>[2x]KKQTQRNVFRCNVIGVKNCGKSGVLQALLGRNLMRQKKIREDHKSYYAINTVYVYGQEKYLLLHDISESEFLTEAEIICDVVCLVYDVSNPKSFEYCARIFKQHFMDSRIPCLIVAAKSDLHEVKQEYSISPTDFCRKHKMPPPQAFTCNTADAPSKDIFVKLTTMAMYPHVTQADLKSSTFLEHHHHHH

Human Miro1 and Miro2 (hMiro1, hMiro2, also called RhoT1 and RhoT2) are MOM protein homologs that play a critical role in mitochondrial trafficking38394041424344. Both associate with Parkin upon mitochondrial depolarization and are ubiquitinated on multiple lysines18374546. Here, we demonstrate that the cGTPase domain is necessary and sufficient for efficient ubiquitination of either hMiro1 or hMiro2 by p-S65 Parkin. We also find that despite considerable similarities between these two substrates, Parkin modifies hMiro1 much more robustly than hMiro2.

To better understand the difference in ubiquitination efficiency between hMiro1 and hMiro2, we first determined the crystal structures of the isolated cGTPase domains of both proteins to high resolution (hMiro1-C: 2.25 Å; hMiro2-C: 1.69 Å). Unexpectedly, both domains crystallized as symmetric dimers. The dimer interface is a highly conserved hydrophobic surface along one face of the cGTPase domain, which, in the intact hMiro1-BC structure, forms the interface with the second hidden EF hand (hEF2). The cGTPase does not mediate dimerization in the context of the full-length molecule, as the hEF2/cGTPase interface is mutually exclusive with cGTPase dimerization, and hMiro1-BC is purely monomeric even at high concentrations. Interestingly, although the same conserved residues mediate dimerization in hMiro1-C and hMiro2-C, their dimer relationships differ significantly. We performed size exclusion chromatography with in-line multi-angle light scattering (SEC-MALS) and confirmed that both hMiro1-C and hMiro2-C dimerize in solution. Subsequently, we successfully disrupted dimerization of hMiro1-C in solution by introducing three mutations at the hydrophobic interface (V418R, Y470S, L472A), thereby generating a stable hMiro1 cGTPase monomer (hMiro1-CM). We note that the two lysines in addition to K572 identified as ubiquitinated by mass spectrometry of the hMiro1-CD, K454 and K512, can be mapped in the dimer, but not the monomer, to roughly the same continuous surface containing K572.>GSHMRKYDVSLTPSGIKVNDEITLLYPALKYAEELYLLINQNKINFIKSMAWPAFVNNISDSVSFIEQSMIDNQNEKALILFIKYKTKIAGVVSFNIIDHANKTAYIGYWLGANFQGKGIVTNAINKLIQEYGDSGVIKRFVIKCIVDNKKSNATALRCGFTLEGVLQKAEILNGVSYDQ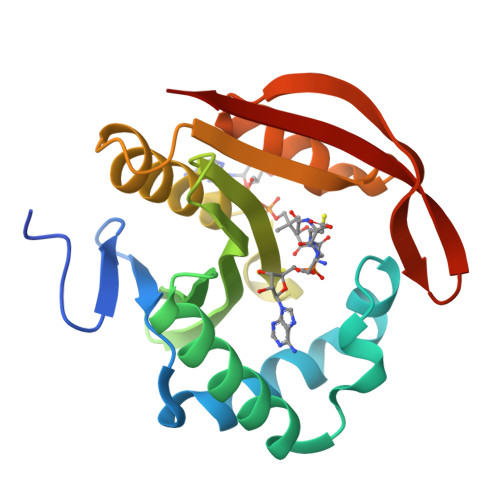NIYSKVIG[2x]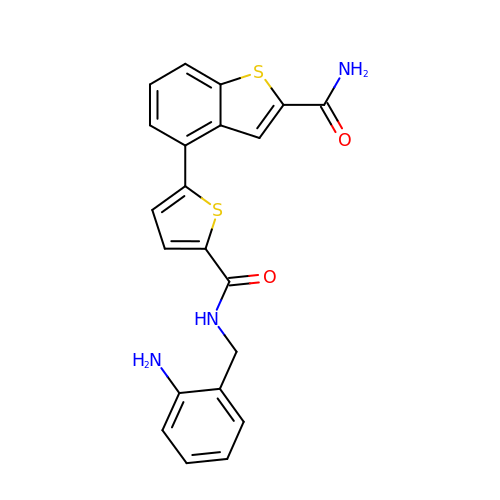4-(5-{[(2-aminophenyl)methyl]carbamoyl}thiophen-2-yl)-1-benzothiophene-2-carboxamide | C21 H17 N3 O2 S2 | UQZFCZAYARDQIK-UHFFFAOYSA-N>[2x]MTSKVYDPEQRKRMITGPQWWARCKQMNVLD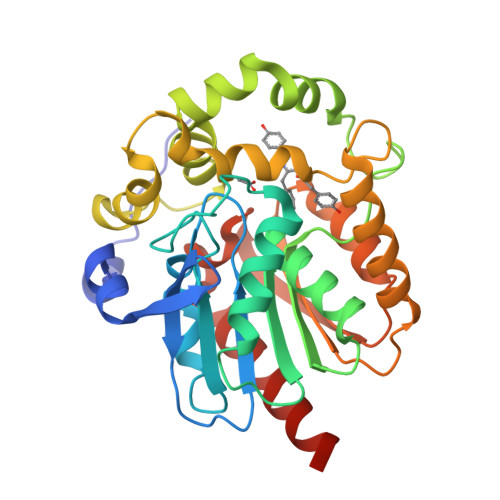SFINYYDSEKHAENAVIFLHGNATSSYLWRHVVPHIEPVARCIIPDLIGMGKSGKSGNGSYRLLDHYKYLTAWFELLNLPKKIIFVGHDFGAALAFHYAYEHQDRIKAIVHMQSVVDVIESWDEWPDIEEDIALIKSEEGEKMVLENNFFVETVLPSKIMRKLEPEEFAAYLEPFKEKGEVRRPTLSWPREIPLVKGGKPDVVQIVRNYNAYLRASDDLPKLFIESDPGFFSNAIVEGAKKFPNTEFVKVKGLHFLQEDAPDEMGKYIKSFVERVLKNEQHHHHHH>[2x]AIHEIKQNGNRYKIEKVTDSSLKQALASLRQSAWNVKELDLSGNPLSQISAADLAPFTKLELLNLSSNVL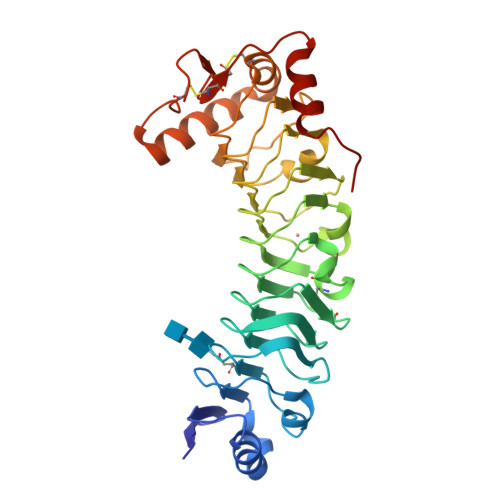YETLDLESLSTLRTLDLNNNYVQELLVGPSIETLHAANNNISRVSCSRGQGKKNIYLANNKITMLRDLDEGCRSRVQYLDLKLNEIDTVNFAELAASSDTLEHLNLQYNFIYDVKGQVVFAKLKTLDLSSNKLAFMGPEFQSAAGVTWISLRNNKLVLIEKALRFSQNLEHFDLRGNGFHCGTLRDFFSKNQRVQTVAKQTVKKLTGQNEEECTVPTLGHYGAYCCEDLPAPFADRLIALGHHHHHH5-methyl-2-(5-methylpyridin-2-yl)pyridine 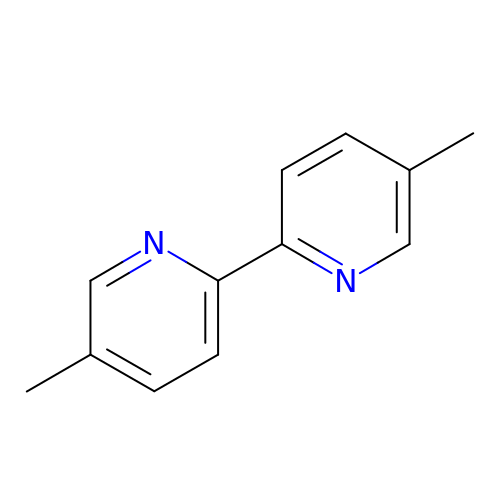| C12 H12 N2 | PTRATZCAGVBFIQ-UHFFFAOYSA-N> MHHHHHHENLYFQSNARVLVVDDDPTCLM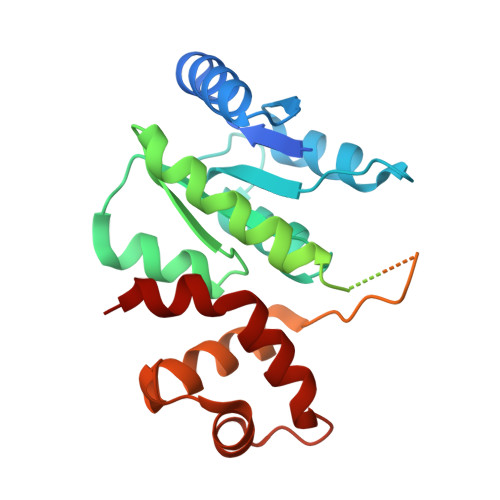ILERMLRTCLYEVTKCNRAEMALSLLRKNKHGFDIVISDVHMPDMDGFKLLEHVGLEMDLPVIMMSADDSKSVVLKGVTHGAVDYLIKPVRMEALKNIWQHVVRKRRSEWSVPEHSGSIEETGERQQQQHRGGGGGAAVSGGEDAVDDNSSSVNEGNNWRSSSRKRKDEEGEEQGDDKDEDASNLKKPRVVWSVELHQQFVAAVNQLGVEKAVPKKILELMNVPGLTRENVASHLQKYRIYLRRLG> MVGFKHTIWALLLMMVTGTAIAQNNTNSPYTRYGYGDLSDQSFGNSKAMGGIAFGLRDGAQINPTNPASYTAIDSLTFLFEGG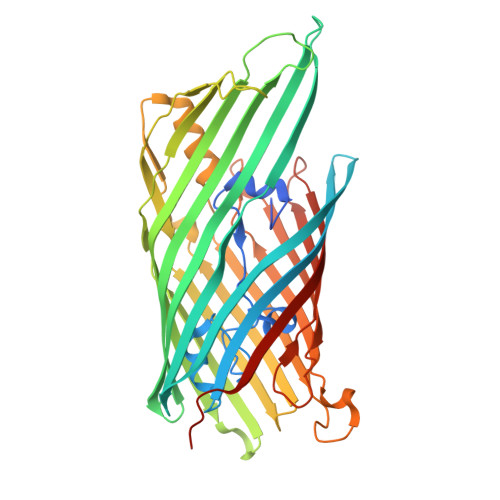VSLQNMNISGGGLKLNAKNASFDYLAMQFRLAPWMAMSVGLLPYSNVGYTVSDSQTTDNGLAYSRSFTGDGGLHQMYVGAGVKVLKNLSVGVNASYFWGDITRTRGMFYPGTSSYDSYQRKMVTSISDYKLDFGAQYTQALNKKSSLTIGAVYSPKHKLNNDYTSIVIMGASSSSYGTEYKDVLDATFELPNTFGVGFTYNYDKRLTVGADYSLQQWSKTNFGVVTSDENVRQDFNETFTYCDRTKISVGAEYIPNLIGRSYFAHIKYRLGAYYTTPYYKIDGKKASREYGVTAGFGLPVPRSRSILSISGQFVRVKGLETNMVNENIFRVSIGLTFNERWFFKRRVE> NEGKALMAIKASFSNVANMLLDWDDVHNHDFCSWRGVFCDNVSLNVVSLNLSNLNLGGEISSALGDLMNLQSIDLQGNKLGGQIPDEIGNCVSLAYVDFSTNLLFGDIPFSISKLKQLEFLNLKNNQLTGPIPATLTQIPNLKTLDLARNQLTGEIPRLLYWNEVLQYLGLRGNMLTGTLSPDMCQLTGLWYFDVRGNNLTGTIPESIGNCTSFEILDVSYNQITGVIPYNIGFLQVATLSLQGNKLTGRIPEVIGLMQALAVLDLSDNELTGPIPPILGNLSFTGKLYLHGNKLTGQIPPELGNMSRLSYLQ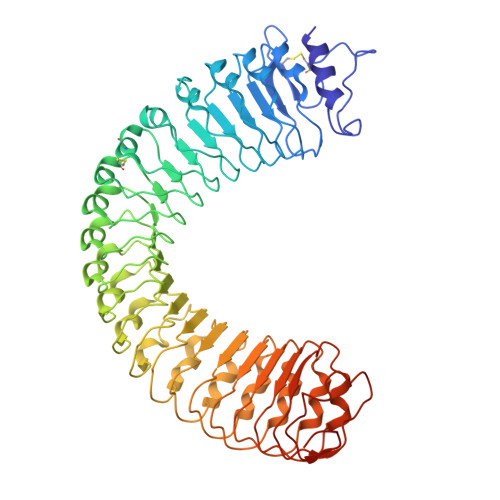LNDNELVGKIPPELGKLEQLFELNLANNNLVGLIPSNISSCAALNQFNVHGNFLSGAVPLEFRNLGSLTYLNLSSNSFKGKIPAELGHIINLDTLDLSGNNFSGSIPLTLGDLEHLLILNLSRNHLNGTLPAEFGNLRSIQIIDVSFNFLAGVIPTELGQLQNINSLILNNNKIHGKIPDQLTNCFSLANLNISFNNLSGIIPPMKNFTRFSPASFFGNPFLCGNWVGSICGPHHHHHH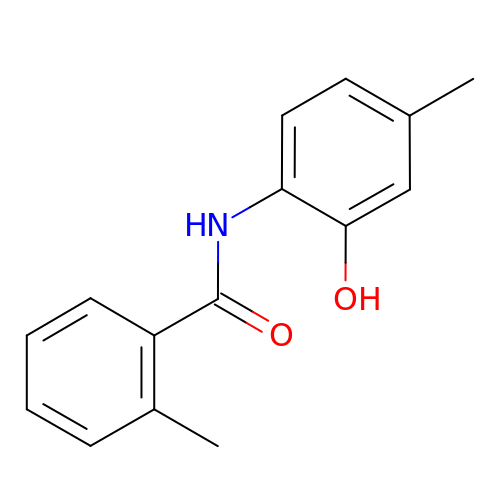N-(2-hydroxy-4-methylphenyl)-2-methylbenzamide | C15 H15 N O2 | JAUMLWIGYIWUPO-UHFFFAOYSA-N5-{4-[(3R)-3-methylmorpholin-4-yl]-6-[1-(S-methylsulfonimidoyl)cyclopropyl]pyrimidin-2-yl}isoquinoline 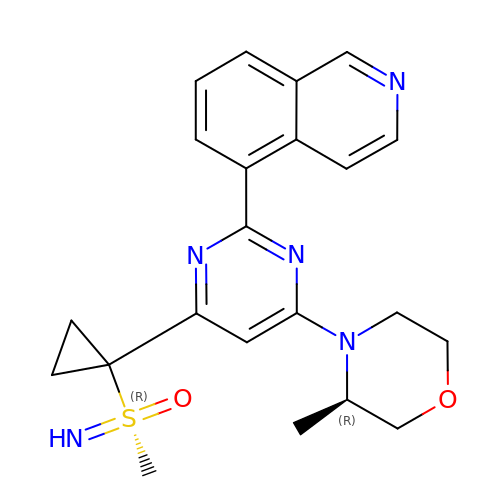| C22 H25 N5 O2 S | QKKJIBZPNHULHG-DHMKHTPVSA-N2-[1,5-dimethyl-2,4-bis(oxidanylidene)-6-(2-oxidanyl-6-oxidanylidene-cyclohexen-1-yl)carbonyl-quinazolin-3-yl]-N-(2-pyren-1-yloxyethyl)ethanamide 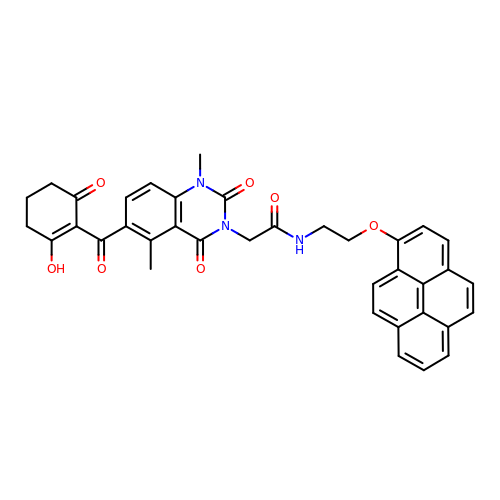| C37 H31 N3 O7 | ILZPFWTUTBFOQA-UHFFFAOYSA-N>GSFTARPSSSMADFRKFFAKAKHIVIISGAGVSAESGVPTFRGAGGYWRKWQAQDLATPLAFAHNPSRVWEFYHYRREVMGSKEPNAGHRAIAECETRLGKQGRRVVVITQNIDELHRKAGTKNLLEIHGSLFKTRCTSCGVVAENYKSPICPALSGKGAPEPGTQDASIPVEKLPRCEEAGCGGLLRPHVVWFGENLDPAILEEVDRELAHCDLCLVVGTSSVVYPAAMFAPQVAARGVPVAE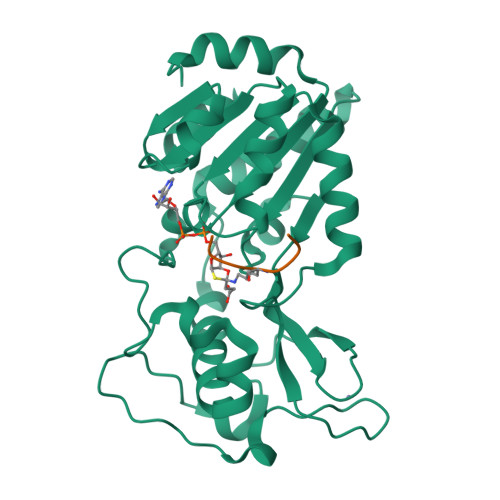FNTETTPATNRFRFHFQGPCGTTLPEALA[2x];>KQTARKSTGGKA[2x]>[8x]MAQLSGQPVVILPEGTQRYVGRDAQRLNILAARIIAETVRTTLGPKGMDKMLVDSLGDIVVTNDCATILDKIDLQHPAAKMMVEVAKTQDKEAGDGTTTAVVIAGELLRKAEELLDQNIHPSIIIKGYALAAEKAQEILDEIAIRVDPDDEETLLKIAATSITGKNAESHKELLAKLAVEAVKQVAEKKDGKYVVDLDNIKFEKKAGEGVEESELVRGVVIDKEVVHPRMPKRVENAKIALINEALEVKKTET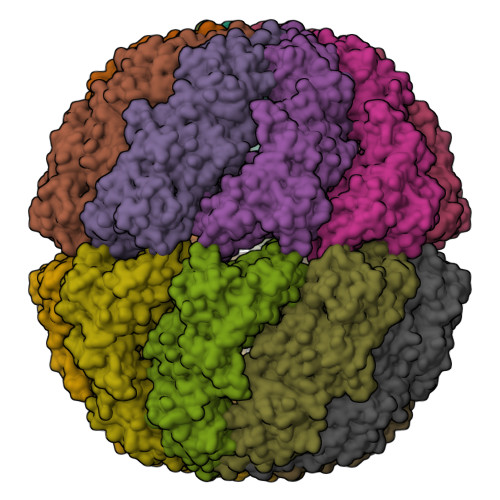DAKINITSPDQLMSFLEQEEKMLKDMVDHIAQTGANVVFVQKGIDDLAQHYLAKYGIMAVRRVKKSDMEKLAKATGAKIVTNVKDLTPEDLGYAEVVEERKLAGENMIFVEGCKNPKAVTILIRGGTEHVIDEVERALEDAVKVVKDVMEDGAVLPAGGAPEIELAIRLDEYAKQVGGKEALAIENFADALKIIPKTLAENAGLDTVEMLVKVISEHKNRGLGIGIDVFEGKPADMLEKGIIEPLRVKKQAIKSASEAAIMILRIDDVIAAKATKPEGGQGGGMPGGMGGMDMGM EcoP15I is a prototype of the Type III R–M family and consists of two methylation (Mod) and one (or two) restriction (Res) subunits, resulting in a Mod2Res1 or Mod2Res2 complex78910. The Mod subunits are responsible for DNA recognition and methylation, while the Res subunits are responsible for ATP hydrolysis and cleavage. Cleavage only occurs if the two recognition sites (CAGCAG) are in an inverted-repeat orientation, arranged either as ‘head-to-head' or ‘tail-to-tail'1112. EcoP15I hydrolyses ∼30 ATP molecules in two steps (a fast consumption of ∼10 ATP molecules followed by a slower consumption of ∼20 ATP molecules), which switches the enzyme into a distinct structural state that can diffuse on DNA over long distances.

We report here the structure of the entire EcoP15I complex (Mod2Res1) bound to its DNA substrate. The EcoP15I holoenzyme was co-crystallized with a 20-mer DNA duplex containing a single EcoP15I recognition site (CAGCAG). The best co-crystals were obtained in the presence of AMP and diffracted to ∼2.6 Å resolution with synchrotron radiation. The refined model consists of two Mod subunits (ModA, residues 13–644; ModB, residues 2–644), one Res subunit (residues 7–810), 20-mer DNA (nucleotides 1–20 on each strand), one AMP molecule, 3 ions and 103 solvent molecules. The EcoP15I Mod2Res1 heterotrimer embraces the DNA duplex and makes extensive protein–DNA contacts. The target adenine (CAGCAG) rotates out of the DNA helix and enters the catalytic pocket of one of the two Mods, ModB. The other Mod, ModA, makes the majority of base-specific contacts with the CAGCAG recognition sequence. Only the helicase core of the Res subunit is visible in the electron density map; the cleavage domain is disordered and may only become ordered when the enzyme collides with another EcoP15I complex and becomes cleavage competent. AMP binds to the ‘bottom' side of the cleft at the confluence of two domains, while the DNA duplex is accommodated on the ‘top' side of the cleft. In particular, proximity of the ModA TRD to the Pin domain in RecA2 suggests a model in which the TRD may switch its location from the DNA major groove to the Pin domain and hence, adopt a ‘nonspecific' conformation more amenable to DNA sliding.

>MKKETIFSEVETANSKQLAVLKANFPQCFDKNGAFIQEKLLEIIRASEVELSKESYSLNWLGKSYARLLANLPPKTLLAEDKTHNQQEENKNSQHLLIKGDNLEVLKHMVNAYAEKVKMIYIDPPYNTGKDGFVYNDDRKFTPEQLSELAGIDLDEAKRILEFTTKGSSSHSAWLTFIYPRLYIARELMREDGTIFISIDHNEFSQLKLVCDEIFGEQNHVGDLVWKNATDNNPSNIAVEHEYIIVYTKNKEQLISEWKSNISDVKNLLVNIGEEFASKYTGNELQEKYTQWFREHRSELWPLDRYKYIDKDGIYTGSQSVHNPGKEGYRYDIIHPKTKKPCKQPLMGYRFPLDTMDRLLSEEKIIFGDDENKIIELKVYAKDYKQKLSSVIHLDGRVATNELKELFPEMTQPFTNAKTIKLVEDLISFACDGEGIVLDFFAGSGTTAHTVFNLNNKNKTSYQFITVQLDEPTKDKSDAMKHGYNTIFDLTKERLIRASKKNRDQGFKVYQLMPDFRAKDESELTLSNHTFFDDVVLTPEQYDTLLTTWCLYDGSLLTTPIEDVDLGGYKAHLCDGRLYLIAPNFTSEALKALLQKVDSDKDFAPNKVVFYGSNFESAKQMELNEALKSYANKKSIELDLVVRN[2x];> MSKGFTLEKNLPHQKAGVDAVMNVFVSATPHLTDNVAVRLLANPELKLSEQQYYNNIKNVQAFNGIAHSKDNHNAKSNIIDVSMETGTGKTYTYIKTIFDLNKSFGINKFIIIVPTLSIKAGTVNFLKSDALKEHFRDDYKRELRTYVVESQKNAGKNTKSYMPQAIHDFVEASNFNKKYIHVLVINSGMINSKSLTDTYDTGLLDNQFNTPVDALRAVKPFIIIDEPHRFPTGKKTWENIEKFNAQYIIRYGATFSEGYKNLVYRLTAVDAFNDDLVKGIDAYIEDIVGDGNANLKFVKSDGKEATFELNENNNKKSFKLAKGESLSKTHSAIHDLTLDALNKSTAVLSNGIELKIGSSINPYSYDQTLADNMMRKAVKEHFKLEKELLTQRPRIKPLTLFFIDDIEGYRDGNDISGSLKTKFEEYVLAEANELLKTEQDAFYKNYLEKTVTNISSVHGGYFSKDNSDKDDKIEQEINEILHDKELLLSLDNPRRFIFSKWTLREGWDNPNVFQICKLRSSGSTTSKLQEVGRGLRLPVNEYMCRVKDRNFTLKYYVDFTEKDFVDSLVKEVNESSFKERVPSKFTQELKEQIMAQYPELSSRALMNELFNDEIIDDNDNFKDSDAYSRLKSKYPAAFPIGVKPGKIKKATDGKRRTKMRVGKFSELKELWDLINQKAVIEYKINSESEFLSIFKSFMLEETERFTKSGVHTRIDKIYIHNDMAMSKSIVSDDDDFAKLNTMSYREFLDNLSQTIFVKHGTLHKVFCDIKDTINITEYLNIQTIRKIKSGFSKYLLNNSFNKFSLGYNLISGSIHPTKFTNADGNPLGEVLSSDLGVLQDNAKAPLDTYLFEEVFYDSELERRNITDREIQSVVVFSKIPKNSIKIPVAGGYTYSPDFAYVVKTAEGDYLNFIIETKNVDSKDSLRLEEKRKIEHAQALFNQISQSVKVEFRTQFANDDIYQLIKSALP>[4x]GSHMQVWPGQA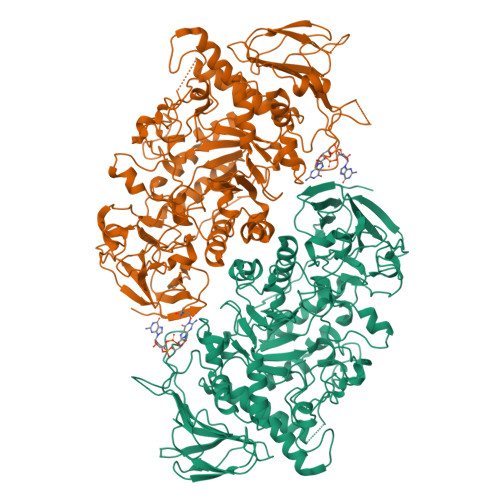YPLGATYDGAGTNFAVFSEAAHRIELCLLHDDGSETAVELRETDAFVRHAYLPGVMPGQRYGFRVHGPYAPERGLRCNAAKLLLDPYARAVSGRVRWGEAVYGYPFGRPDARNDLDSAPDTMTSVVVNPYFDWGDDRRPRTEYHHTVIYEAHVKGLTMLHPDLPEELRGTYAGLAHPSVIGHLRELGVTALELMPVHQFVNDHRLVDAGLSNYWGYNTIGFFAPHNAYASWGDRGQQVLEFKSAVRALHQAGIEVILDVVYNHTAEGNHLGPTLSMRGLDNPSYYRLADDPRYYMDTTGTGNSLLMRSPHVLQLIMDSLRYWVTEMHVDGFRFDLAATLARQFHEVDRLSSFFDLVQQDPVVSQVKLIAEPWDVGEGGYQVGNFPPLWTEWNGKYRDCVRDLWRGEPRTLAEFASRLTGSSDLYQDDGRRPLASVNFVTCHDGFTLRDLVSYNEKRNEANGEGNRDGENYNRSWNCGEEGETEDVGITELRARQMRNFLATLMLSQGVPMLSHGDEFGRTQGGNNNAYCQDNEVSWVRWPKENSEAEATLLRFTRSMVRLRREHPVFRRRRFFHGRPVEGTHDELTDIAWFTPEGEEMTSRDWQAAHAQALTVFLNGNAISEPGTQGERIADDSFLLMFNASAKELEFVVPDSHGRYWRMVVDTSDPEGMPPQQGPELAGGERVTLAPLSLTVLRRPA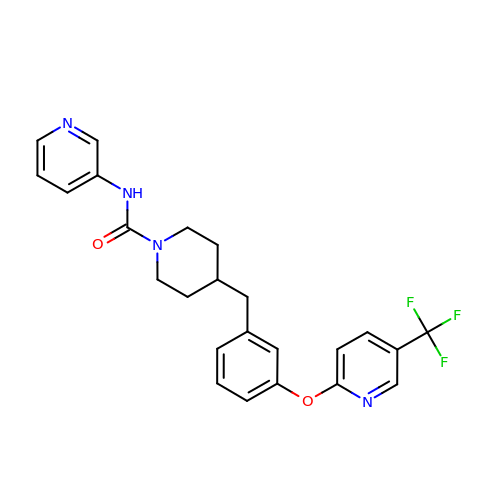N-pyridin-3-yl-4-[[3-[5-(trifluoromethyl)pyridin-2-yl]oxyphenyl]methyl]piperidine-1-carboxamide | C24 H23 F3 N4 O2 | NBOJHRYUGLRASX-UHFFFAOYSA-N>[8x]MQEKPQEPKVVGVEILEKSGLDIKKLVDKLVKATAAEFTTYYYYTI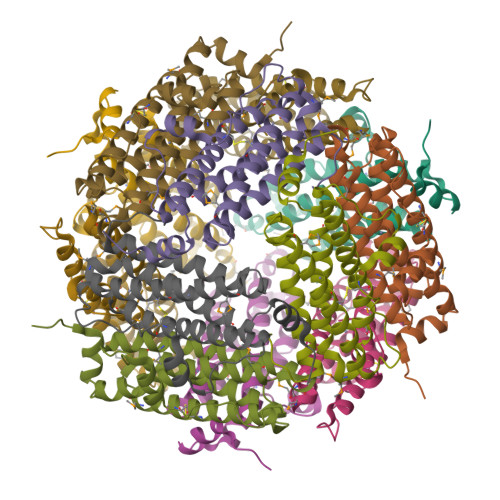LRMHLTGMEGEGLKEIAEDARLEDRLHFELMTQRIYELGGGLPRDIRQLADISACSDAYLPENWKDPKEILKVLLEAEQCAIRTWKEVCDMTYGKDPRTYDLAQRILQEEIEHEAWFLELLYGRPSGHFRRSSPGNAPYSKK Transcription elongation stalls at lesions in the DNA template. RNA polymerase (RNAP) may pause on encountering lesions in the DNA template that result from ionizing radiation, ultraviolet (UV) irradiation, and chemical and enzymatic reactions. Here we show that translation, which is coupled to transcription in bacteria, actively dislodges stalled ECs from the damaged DNA template. Our results indicate that coupled ribosomes functionally and kinetically discriminate between paused ECs and stalled ECs, ensuring the selective destruction of only the latter.

To understand the possible reasons for stalled EC vulnerability to ribosome-mediated destruction, we determined the structure of the EC stalled at the T=T dimer (ECT=T) after incorporation of adenosine monophosphate (AMP) at the first T of the lesion using cryogenic electron microscopy (cryo-EM). ECs were obtained by walking as above. We obtained a uniform set of particles, which did not yield more distinct states during classification. Despite an observed orientation bias, the structure was solved to 2.9 Å resolution. As expected, the arrangement of nucleic acids in the active site corresponded to the analogous structure of eukaryotic RNAP II stalled after incorporation of AMP at the T=T dimer (post-translocated RNAP II ECT=T in Extended Data Fig. 8c). Notably, the β′ clamp of the stalled EC was in the closed (but not swivelled) conformation. Indeed, we observed that a stalled EC was much more sensitive to the high salt treatment than a paused EC. Although the overall structures of paused and stalled ECs are similar, the local differences in the position of the damaged nucleic acids within the stalled EC is probably responsible for its vulnerability to being dislodged by a coupled ribosome. We proposed that the vulnerability of the stalled EC to ribosome dismissal may be dictated by the Trigger Loop, which may ‘feel’ the unusual arrangement of nucleic acids. We, however, cannot interpret these findings on the basis of the ECT=T structure, as the Trigger Loop was not resolved in it.

>[2x]MQGSVTEFLKPRLVDIEQVSSTHAKVTLEPLERGFGHTLGNALRRILLSSMPGCAVTEVEIDGVLHEYSTKEGVQEDILEILLNLKGLAVRVQGKDEVILTLNKSGIGPVTAADITHDGDVEIVKPQHVICHLTDENASISMRIKVQRGRGYVPASTRIHSEEDERPIGRLLVDACYSPVERIAYNVEAARVEQRTDLDKLVIEMETNGTIDPEEAIRRAATILAEQLEAFVDLRVLFQ;> MVYSYTEKKRIRKDFGKRPQVLDVPYLLSIQLDSFQKFIEQDPEGQYGLEAAFRSVFPIQSYSGNSELQYVSYRLGEPVFDVQECQIRGVTYSAPLRVKLRLVIYEREAPEGTVKDIKEQEVYMGEIPLMTDNGTFVINGTERVIVSQLHRSPGVFFDSDKGKTHSSGKVLYNARIIPYRGSWLDFEFDPKDNLFVRIDRRRKLPATIILRALNYTTEQILDLFFEKVIFEIRDNKLQMELVPERLRGETASFDIEANGKVYVEKGRRITARHIRQLEKDDVKLIEVPVEYIAGKVVAKDYIDESTGELICAANMELSLDLLAKLSQSGHKRIETLFTNDLDHGPYISETLRVDPTNDRLSALVEIYRMMRPGEPPTREAAESLFENLFFSEDRYDLSAVGRMKFNRSLLREEIEGSGILSKDDIIDVMKKLIDIRNGKGEVDDIDHLGNRRIRSVGEMAENQFRVGLVRVERAVKERLSLGDLDTLMPQDMINAKPISAAVKEFFGSSQLSQFMDQNNPLSEITHKRRISALGPGGLTRERAGFEVRDVHPTHYGRVCPIETPEGPNIGLINSLSVYAQTNEYGFLETPYRKVTDGVVTDEIHYLSAIEEGNYVIAQANSNLDEEGHFVEDLVTCRSKGESSLFSRDQVDYMDVSTQQVVSVGASLIPFLEHDDANRALMGANMQRQAVPTLRADKPLVGTGMERAVAVDSGVTAVAKRGGVVQYVDASRIVIKVNEDEMYPGEAGIDIYNLTKYTRSNQNTCINQMPCVSLGEPVERGDVLADGPSTDLGELALGQNMRVAFMPWNGYNFEDSILVSERVVQEDRFTTIHIQELACVSRDTKLGPEEITADIPNVGEAALSKLDESGIVYIGAEVTGGDILVGKVTPKGETQLTPEEKLLRAIFGEKASDVKDSSLRVPNGVSGTVIDVQVFTRDGVEKDKRALEIEEMQLKQAKKDLSEELQILEAGLFSRIRAVLVAGGVEAEKLDKLPRDRWLELGLTDEEKQNQLEQLAEQYDELKHEFEKKLEAKRRKITQGDDLAPGVLKIVKVYLAVKRRIQPGDKMAGRHGNKGVISKINPIEDMPYDENGTPVDIVLNPLGVPSRMNIGQILETHLGMAAKGIGDKINAMLKQQQEVAKLREFIQRAYDLGADVRQKVDLSTFSDEEVMRLAENLRKGMPIATPVFDGAKEAEIKELLKLGDLPTSGQIRLYDGRTGEQFERPVTVGYMYMLKLNHLVDDKMHARSTGSYSLVTQQPLGGKAQFGGQRFGEMEVWALEAYGAAYTLQEMLTVKSDDVNGRTKMYKNIVDGNHQMEPGMPESFNVLLKEIRSLGINIELEDE;> MKDLLKFLKAQTKTEEFDAIKIALASPDMIRSWSFGEVKKPETINYRTFKPERDGLFCARIFGPVKDYECLCGKYKRLKHRGVICEKCGVEVTQTKVRRERMGHIELASPTAHIWFLKSLPSRIGLLLDMPLRDIERVLYFESYVVIEGGMTNLERQQILTEEQYLDALEEFGDEFDAKMGAEAIQALLKSMDLEQECEQLREELNETNSETKRKKLTKRIKLLEAFVQSGNKPEWMILTVLPVLPPDLRPLVPLDGGRFATSDLNDLYRRVINRNNRLKRLLDLAAPDIIVRNEKRMLQEAVDALLDNGRRGRAITGSNKRPLKSLADMIKGKQGRFRQNLLGKRVDYSGRSVITVGPYLRLHQCGLPKKMALELFKPFIYGKLELRGLATTIKAAKKMVEREEAVVWDILDEVIREHPVLLNRAPTLHRLGIQAFEPVLIEGKAIQLHPLVCAAYNADFDGDQMAVHVPLTLEAQLEARALMMSTNNILSPANGEPIIVPSQDVVLGLYYMTRDCVNAKGEGMVLTGPKEAERLYRSGLASLHARVKVRITEYEKDANGELVAKTSLKDTTVGRAILWMIVPKGLPYSIVNQALGKKAISKMLNTCYRILGLKPTVIFADQIMYTGFAYAARSGASVGIDDMVIPEKKHEIISEAEAEVAEIQEQFQSGLVTAGERYNKVIDIWAAANDRVSKAMMDNLQTETVINRDGQEEKQVSFNSIYMMADSGARGSAAQIRQLAGMRGLMAKPDGSIIETPITANFREGLNVLQYFISTHGARKGLADTALKTANSGYLTRRLVDVAQDLVVTEDDCGTHEGIMMTPVIEGGDVKEPLRDRVLGRVTAEDVLKPGTADILVPRNTLLHEQWCDLLEENSVDAVKVRSVVSCDTDFGVCAHCYGRDLARGHIINKGEAIGVIAAQSIGEPGTQLTMRTFHIGGAASRAAAESSIQVKNKGSIKLSNVKSVVNSSGKLVITSRNTELKLIDEFGRTKESYKVPYGAVLAKGDGEQVAGGETVANWDPHTMPVITEVSGFVRFTDMIDGQTITRQTDELTGLSSLVVLDSAERTAGGKDLRPALKIVDAQGNDVLIPGTDMPAQYFLPGKAIVQLEDGVQISSGDTLARIPQESGGTKDITGGLPRVADLFEARRPKEPAILAEISGIVSFGKETKGKRRLVITPVDGSDPYEEMIPKWRQLNVFEGERVERGDVISDGPEAPHDILRLRGVHAVTRYIVNEVQDVYRLQGVKINDKHIEVIVRQMLRKATIVNAGSSDFLEGEQVEYSRVKIANRELEANGKVGATYSRDLLGITKASLATESFISAASFQETTRVLTEAAVAGKRDELRGLKENVIVGRLIPAGTGYAYHQDRMRRRAAGEAPAAPQVTAEDASASLAELLNAGLGGSDNE;> MARVTVQDAVEKIGNRFDLVLVAARRARQMQVGGKDPLVPEENDKTTVIALREIEEGLINNQILDVRERQEQQEQEAAELQAVTAIAEGRR> ALLTFFATDARLDPAEQDRLFRRVMDRTFNAVSIDTDTSTSDTAVLFANGLAGEVDAGEFEEALHTAALALVKDIASDGEGAAKLIEVQVTGARDDAQAKRVGKTVVNSPLVKTAVHGCDPNWGRVAMAIGKCSDDTDIDQERVTIRFGEVEVYPPKARGDQADDALRAAVAEHLRGDEVVIGIDLAIADGAF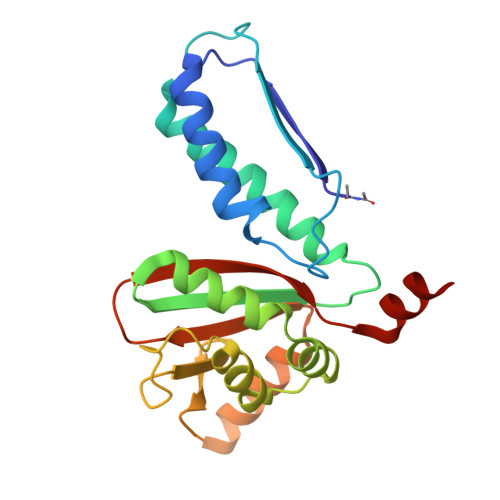TVYGCDLTEGYVRLNSEYTT>GSMPMYEVQWKVVEESNGNNYSYIDPTQLPYDHKWEFPRNRLSFGKTLGAGAFGKVVEATAQGLIKSDAAMTVAVKMLKPSAHSTEREALMSELKVLSYLGNHENIVNLLGACTHGGPTLVIIEYCCYGDLLNFLRRKRDEFVPYKVAPEDLYKDFLTLEHLLSFSYQVAKGMAFLASKNCIHRDLAARNILLTHGNITKICDFGLARDIKNDSNYVDKGNARLPVKWMAPESIFNSVYTFESDVWSYGIFLWELFSLGSSPYPGMPVDSKFYKMIKEGFRMSSPEYAPAEMYDIMKTCWDADPDKRPTFKQIVQDIEKQISESTNH[2x]

Avapritinib is the only potent and selective inhibitor approved for the treatment of D842V-mutant gastrointestinal stromal tumors (GIST), the most common primary mutation of the platelet-derived growth factor receptor α (PDGFRA). Against this background, we solve the crystal structures of avapritinib in complex with wild-type and mutant PDGFRA and stem cell factor receptor (KIT), which provide evidence and understanding of inhibitor binding and lead to the identification of a sub-pocket (Gα-pocket). Furthermore, we report the identification of a sub-pocket (Gα-pocket) located in the N-lobe of the kinase domain, which is surrounded by amino acids of key regulatory elements such as the Gly-rich loop and the αC-helix.

Intense screening and optimization resulted in two complex structures with avapritinib in wt and gatekeeper-mutant KIT-T670I. To the best of our knowledge, this is the first report of a structure of T670I mutated KIT. In contrast, in the T670I-mutated kinase, this position is occupied by the isoleucine side chain, and no water-mediated contact can be observed. Additionally, the introduced hydrophobic isoleucine is close to the polar scaffold, presumably contributing to a reduced binding affinity. Based on their MD simulation, Winger et al. suggested that the T670I mutation confers resistance via distant conformational changes within the Gly-rich loop, which we cannot confirm based on our complex crystal structures.> MPKTGREKRKSPENRFLRKLLKPDIERERLKAVNSIISIVFGTRRIAWAHLDRKLTVLDWQQ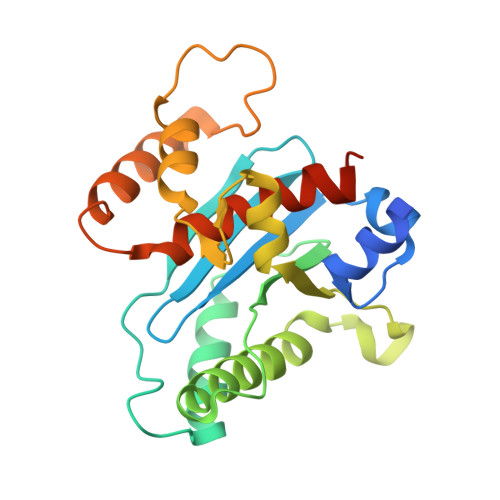SDRWSLMRGIYSSSVYLEEISSIISKMPKADFYVLEKTGLSIQNSSLFPILLHFHIMEAMLYALLNKTFAQDGQHQVLSMNRNAVGKHFELMIGDSRTSGKELVKQFLFDSILKADPRVFFPSDKIVHYRQMFLSTELQRVEELYDSLLQAIAFYELAVFDSQPLEHHHHHH>[2x]GGSVIVIDSKAAWDAQLAKGKEEHKPIV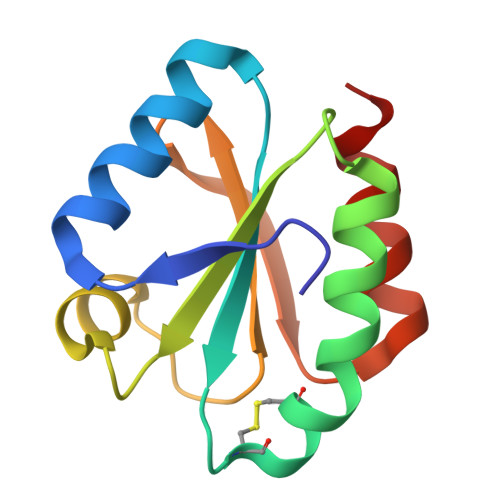VAFTATWCGPCKMIAPLFETLSNDYAGKVIFLKVDVDAVAAVAEAAGITAMPTFHVYKDGVKADDLVGASQDKLKALVAKHAAA> MENQILTQLYGRGWAFPPVFSLEKGVEMAEGAEDVRQSLQILFSTEPGERLMRENYGCGLNDF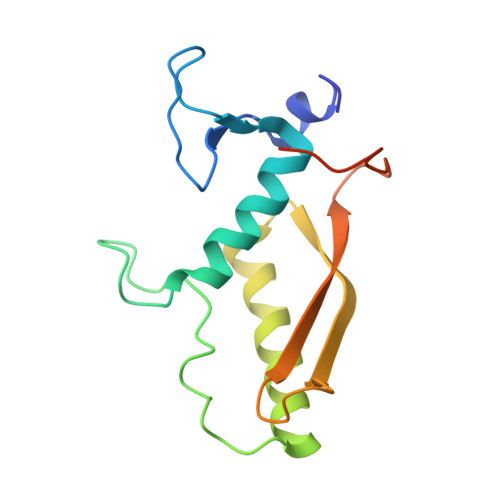MFENIRNELIAEIESHIHDNVLRYEPRADMTDIQVRQSPGMGNTLQVQVMYRLRGSDINQQIQGVLALSEGRVTEVV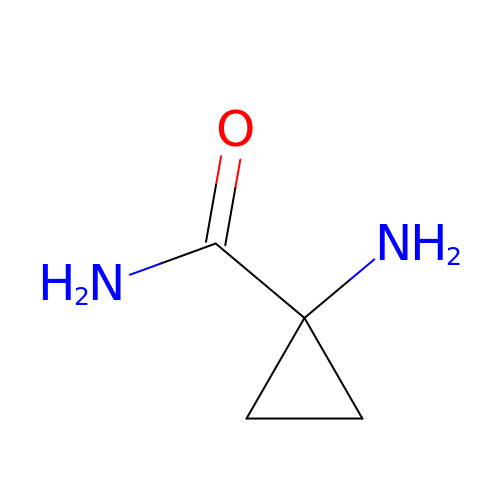1-aminocyclopropane-1-carboxamide | C4 H8 N2 O | JFGXRDGYMLGBBB-UHFFFAOYSA-N>PPGTVDKKMVEKCWKLMDKVVRLCQNPKLALKNSPPYILDLLPDTYQHLRTILSRYEGKMETLGENEYFRVFMENLMKKTKQTISLFKEGKERMYEENSQPRRNLTKLSLIFSHMLAELKGIFPSGLFQGDTFRITKADAAEFWRKAFGEKTIVPWKSFRQALHEVHPISSGLEAMALKSTIDLTCNDYISVFEFDIFTRLFQPWSSLLRNWNSLAVTHPGYMAFLTYDEVKARLQKFIHKPGSYIFRLSCTRLGQWAIGYVTADGNILQTIPHNKPLFQALIDGFREGFYLFPDGRNQNPDLTGLCEPTPQDHIKVTQEQYELYCEMGSTFQLCKICAENDKDVKIEPCGHLMCTSCLTSWQESEGQGCPFCRCEIKGTEPIVVDPFD[2x];>[2x]TLNSDGYTP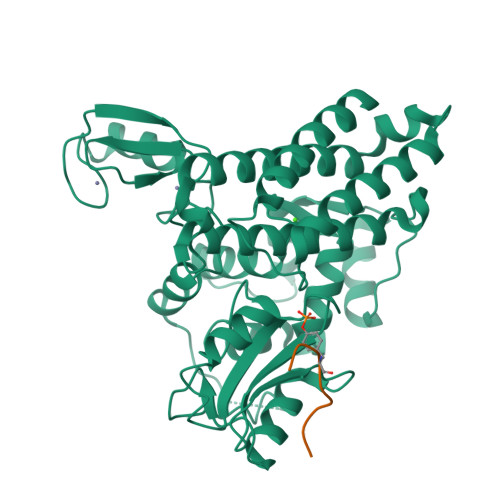EPA>XGELAQSLKEL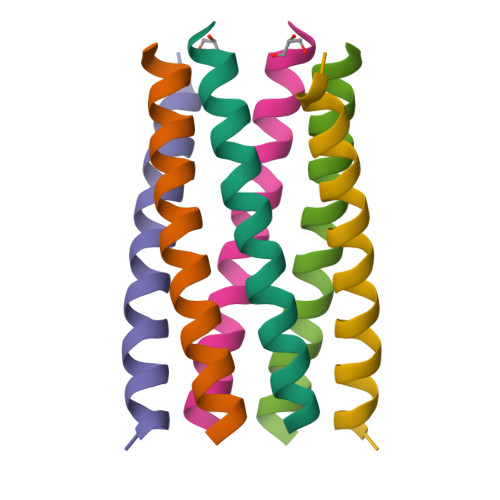AKSLKELAWSLKELAQSLKGX[3x]>GPGSLSQASADLEATLRHKLTVMYSQINGASRALDDVRNRQQDVRMTANRKVEQLQQEYTEMKALLDASETTSTRKIKEEEKRVNSKFDTIYQILLKKKSEIQTLKEEIEQSLTKRDEFEFLEKASKLRGISTKPVYIPEVELNHKLIKGIHQSTIDLKNELKQCIGRLQELTPSSGDPGEHDPASTHKSTRP[4x];>GPGMDPNTVSSFQVDCFLWHVRKRVADQELGDAPFLDRLRADQASLRGRGSTLGLDIETATRAGKQIVERILKEESDEALKMTMASVPASRYLTDMTLEEMSREWSMLIPKQKVAGPLCIRMDQAIMDKNIILKANFSVIFDRLETLILLRAFTEEGAIVGEISPLPSLPGHTAE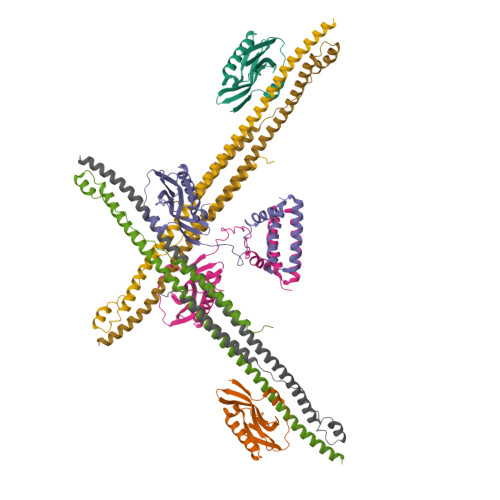DVKNAVGVLIGGLEANDNTVRVSETLQRFAWRSSNENGRPPLTPKQKREMAGTIRSEV[4x]>[2x]GGRAGVESGLSSIETVAAEGRGGYLLREQLDDALAHRQGSPAAYKLYLSVNEQRFARGVRLDNVANRFELRMSVDWRLLDAKNGAEVHKGRTDVSVTYDSADQPYAAIAAQQDGQERAAAE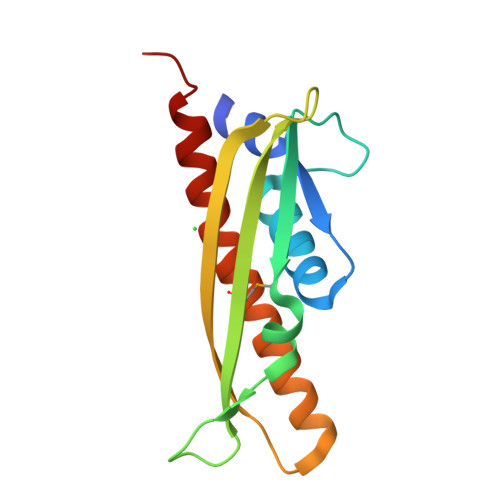AARKIQLDLATWLAGKKPA>[4x]MGHHHHHHHHHHS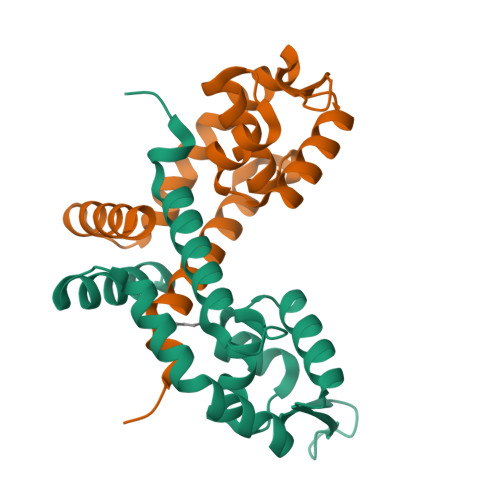SGHIDDDDKHTSLEVLFQGPHMPASQDKLDVPPGPYHFSEQVGHLLRRAYQRHVAIFQQTIPDSKLTAAQFVVLCALRDQGACSLVDVVKATAIDQATVRGVIERLKARKLLAVSHDPADRRKVLVTLTPDGRALVEEMVPFAEQITQSTFGGLNPAERVAIVYLLRKMSDADDLVGRQSDS>SDEVRKNLMDMFRDRQAFSEHTWKM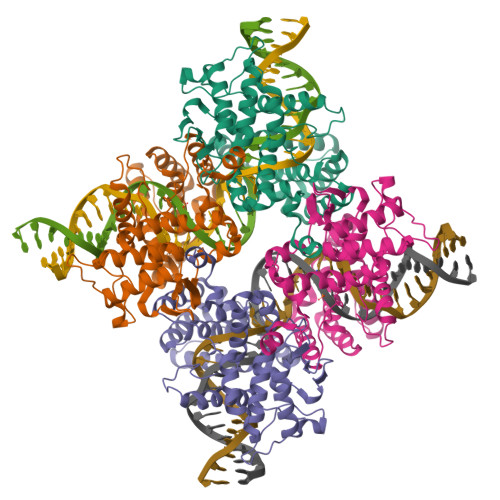LLSVCRSWAAWCKLNNRKWFPAEPEDVRDYLLYLQARGLAVKTIQQHLGQLNMLHRRSGLPRPSDSNAVSLVMRRIRKENVDAGERAKQALAFERTDFDQVRSLMENSDRCQDIRNLAFLGIAYNTLLRIAEIARIRVKDISRTDGGRMLIHIGRTKTLVSTAGVEKALSLGVTKLVERWISVSGVADDPNNYLFCRVRKNGVAAPSATSQLSTRALEGIFEATHRLIYGAKDDSGQRYLAWSGHSARVGAARDMARAGVSIPEIMQAGGWTNVNIVMNYIRNLDSETGAMVRLLED[4x]>[2x]MRKAAGKYGNTLEFGHLVGGEEVLEGPLLERRNPSDREDVVARFPEADKDLVRKAALKAREAFAEWSRTPAPIRGQVLFNLVKILEREKPTLTRLMVREVGKTPKEAAGDVQEAIDTALFFASEGRRLYGQTVPSEMRDKELFTFRRPLGVVGIITAGNFPIAVPSWKLIPAVLTGNTVVWKPSEDAPTLSFVFAKLFEEAGLPPGVLNVVFGGGKGSTGQWMVELMDEGLFQKFAFTGSTQVGRWIGEVAGRNLIRPTLELGGKNPLVVMRDADLDLAVEGAWWSAFATGGQRCTSAGNILVDAPIYEEFKRRFLERVEATLVGNPLLHPEVTYGPFINERFFARWQEHYRVGEAEGARLLFGRGRITRENPYPRFLGDPEAGLYGWPTVWEVRPGTRLFTEEVFGPTINLVKVDGIEEAIAVANSTPYGLSSAIYTNHRHWAYLFKVGIRAGMTSINNATVGAEAHLPFGGVKASGNGGRESGIWVLEEYTYWHAVNEEYSGRLQLAQMDTGYVSPKAPTPWGEVLGL

Found in both prokaryotes and eukaryotes, aldehyde dehydrogenases (ALDH) (EC 1.2.1.3) constitute a large family of NAD(P)-dependent enzymes with molecular weights of 50–60 kDa. ALDHTt contains an unusually extended C-terminal arm forming novel interactions with the N-terminus in the quaternary structure which interacts closely with the substrate entry tunnel. The ALDHTt monomer is composed of the three domains common to all ALDHs: (i) The NAD(P)+ binding domain (1–125 + 148–261) comprising a Rossman fold, (ii) the catalytic domain (267–458) and (iii) the oligomerization domain (126–147 + 494–501). However, the presence in ALDHTt of an unusual extended arm that wrap the facing monomer through H-bonds and salt bridges shows for the first time how the tetramer is not merely a dimer-of-dimers carrying out their functions independent of each other, but that the interaction of the N- and C-termini in CS-related monomers may regulate active site access in NCS-related molecules.

Initially, when we solved the structure of the native ALDHTt, we noticed the presence of an extended C-terminal tail. However, in the native structure, Glu261 has the “In” conformation, associated with proton abstraction from the thiol prior to substrate binding. As previously observed in the human ALDH2 and Ct-FDH structures, Glu261 is suitably oriented and within a short distance to Cys295 to act as a general base for its activation. In addition, the catalytic Cys295 side chain of the native structure is observed in two different conformations, the “attacking” conformation and the “resting” conformation where the side chain is rotated away from the Glu261. In the native crystal structure two partially occupied and mutually exclusive n-octyl-β-glucoside (BOG) molecules originating from the detergent used for caa3-oxidase purification; are found deep within the centre of the tetramer. They lie in a highly positive pore created by the oligomerisation domain and inter-domain linkers of each monomer. There is hydrogen bonding between the head group of the BOG and the positively charged sidechain of Arg127 on the junction between the oligomerisation domain and cofactor binding domain which is positioned directly beside Arg126 which we believe to play a crucial role in tail orientation and thus active site access. Another intriguing observation with ALDHTt is the presence of BOG molecules at the dimer-dimer interface. These BOG molecules have been modelled at partial occupancy which suggests that the detergent molecules sample several conformations in the tetramer’s pore. The negative head group of the detergent molecule is attracted to this charged pore and then becomes trapped in the central cavity. It is tempting to postulate that this highly charged pore is not coincidental and that this is a possible allosteric regulation site for ALDHTt which allows access to the substrate tunnel of each monomer.>MALSANSDAVTYAKAANTRTAAETGDRIEWVKLSLAFLPLATPVSDAKVLTGRQKPLTEVAIIIAEIRSRDGFEGVGFSYSKRAGGQGIYAHAKEIADNLLGEDPNDIDKIYTKLLWAGASVGRSGMAVQAISPIDIALWDMKAKRAGLPLAKLLGAHRDSVQCYNTSGGFLHTPLDQVLKNVVISRENGIGGIK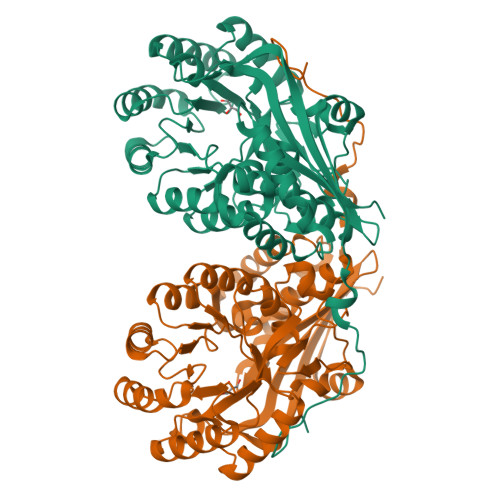LKVGQPNCAEDIRRLTAVREALGDEFPLMVDANQQWDRETAIRMGRKMEQFNLIWIEEPLDAYDIEGHAQLAAALDTPIATGEMLTSFREHEQLILGNASDFVQPDAPRVGGISPFLKIMDLAAKHGRKLAPHFAMEVHLHLSAAYPLEPWLEHFEWLNPLFNEQLELRDGRMWISDRHGLGFTLSEQARRWTQLTCEFGKRP[3x]> SMIKSYAAKEAGGELEVYEYDPGELRPQDVEVQVDYCGICHSDLSMIDNEWGFSQYPLVAGHEVIGRVVALGSAAQDKGLQVGQRVGIGWTARSCGHCDACISGNQINCEQGAVPTIMNRGGFAEKLRADWQWVIPLPENIDIESAGPLLCGGITVFKPLLMHHITATSRVGVIGIGGLGHIAIKLLHAMGCEVTAFSSNPAKEQEVLAMGADKVVNSRDPQALKALAGQFDLIINTVNVSLDWQPYFEALTYGGNFHTVGAVLTPLSVPAFTLIAGDRSVSGSATGTPYELRKLMRFAARSKVAPTTELFPMSKINDAIQHVRDGKARYRVVLKA;> MIKSYAAKEAGGELEVYEYDPGELRPQDVEVQVDYCGICHSDLSMIDNEWGFSQYPLVAGHEVIGRVVALGSAAQDKGLQVGQRVGIGWTARSCGHCDACISGNQINCEQGAVPTIMNRGGFAEKLRADWQWVIPLPENIDIESAGPLLCGGITVFKPLLMHHITATSRVGVIGIGGLGHIAIKLLHAMGCEVTAFSSNPAKEQEVLAMGADKVVNSRDPQALKALAGQF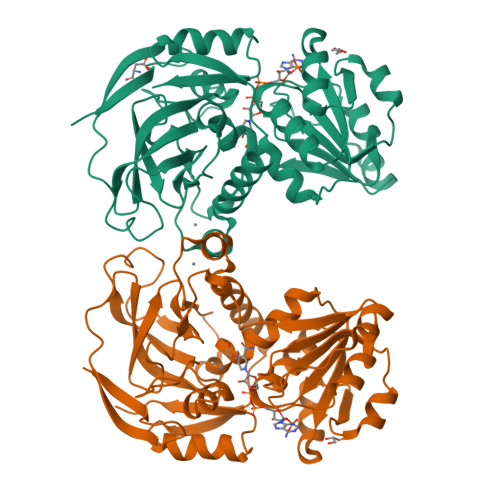DLIINTVNVSLDWQPYFEALTYGGNFHTVGAVLTPLSVPAFTLIAGDRSVSGSATGTPYELRKLMRFAARSKVAPTTELFPMSKINDAIQHVRDGKARYRVVLKADY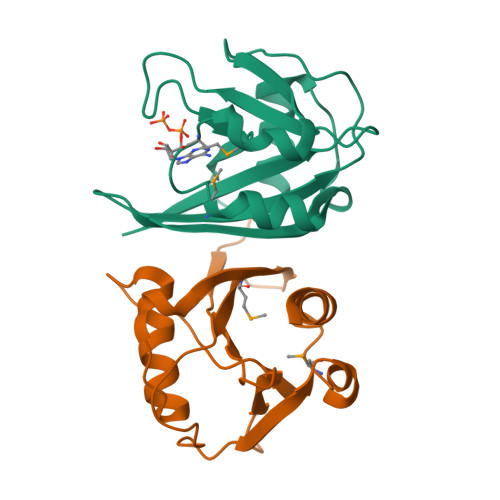>MSLGLPILLVTAAALIDPDGRVLLAQRPPGKSLAGLWEFPGGKLEPGETPEAALVRELAEELGVDTRASCLAPLAFASHSYDTFHLLMPLYACRSWRGRATAREGQTLAWVRAERLREYPMPPADLPLIPILQDWLEGHHHHHH[2x]>MLAGSVQTRHDLLQGAQILVNQVGYHPATPKQAVLALAPGTAAGIRPGWTPTLQIVRADDGQVVWEGTMAGPSEDRLVSGDTLYRADFTSLTAPGRYVAQVVGGPRSPEFAIGPVYRDVLYAAARSYYLQRCGVAIDDPITGVSHALDHHEDGYVLVDDPFYRAGTRLEATGGWHDAGDYGKYVTTTAVTAAQLLKAYELYPQAFADGQLHLPESGNGVPDILDEVRWGLEWLFRMQRPDGAVYHKLAGLRWPGMIRPEQDVQRRYVYRITTQDTAKAAAAWAMAARIFAPFDAAFARKALAAAEQAWRFLAASGPILDYPAEDNSGSGPYDDRDDADDRFWAAVELWVVTGRAEYHDYIARMARTGLPAYAPVSWVNPAALGYFDYVTLGQKGDPAIRARLVQRILEGARSVFQTYEQSGYGVPILAGSFHWGSNKEALAKGMLLLFAHHLEPRPEYERAALAQLDYV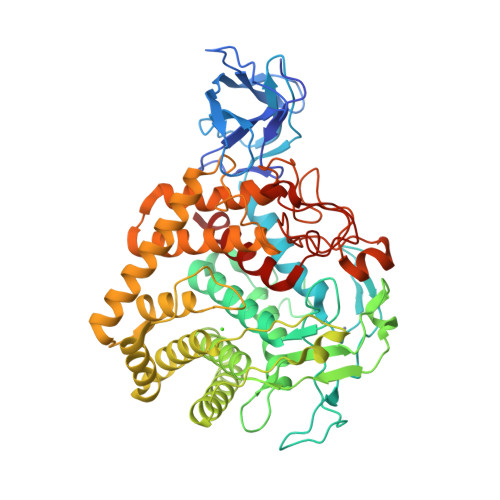LGVNPLAKSYVTGLGSNPPRNPHHRLVKASGVMVPGLLVGGPNDHPQTKAIRPHMGPRGYADVTDSYETNEPAIDYNAPLVFVAAHFASL[2x]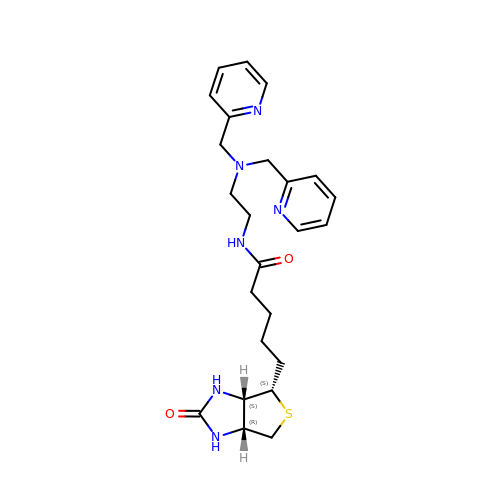N-(2-{bis[(pyridin-2-yl)methyl]amino}ethyl)-5-[(3aS,4S,6aR)-2-oxohexahydro-1H-thieno[3,4-d]imidazol-4-yl]pentanamide | C24 H32 N6 O2 S | GXLJCVSDSFWSLD-FUDKSRODSA-N>[4x]MDAKARNCLLQHREALEKDIKTSYIMDHMISDGFLTISEEEKVRNEPTQQQRAAMLIKMILKKDNDSYVSFYNAL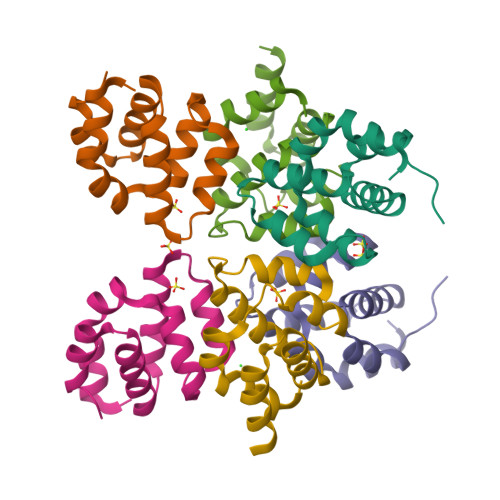LHEGYKDLAALLHDGIPVVSSS;>MDEADRRLLRRCRLRLVEELQVDQLWDALLSRELFRPHMIEDIQRAGSGSRRDQARQLIIDLETRGSQALPLFISCLEDTGQDMLASFLRTNRQAAKLSKLEHHHHHH[2x]To translocate on solid surfaces many bacteria use dynamic cell surface structures called type IVa pili (T4aP). T4aP undergo cycles of extension, adhesion to a surface, and retraction that generate a force sufficient to pull a cell forward. The T4aP filament is composed of thousands of copies of the major pilin. Here, using cryo-EM, we solve the structure of the T4aP of Myxococcus xanthus (T4aPMx), which has an unusual large major pilin called PilA.

For structure determination of T4aPMx, we purified T4aP from the hyperpiliated ΔpilT strain, in which T4aP are extended but not retracted, thereby allowing the purification of T4aP of sufficient purity and quantity for structural analyses. We used cryo-EM to determine the structure of the T4aPMx and obtained the structure at 3.0 Å resolution, the highest resolution so far reported for a T4aP structure. The subunits in the filament are related to each other by an azimuthal rotation of 100.7° and an axial rise per subunit of 10.0 Å, generating a right-handed 1-start helix with a pitch of ~36 Å and 3.6 subunits per turn, as determined from the power spectrum of the filaments. The filaments are ~7 nm in diameter and, in contrast to all previous T4aP structures, resemble a rather solid cylinder without the corrugation of the surface observed in other T4aP structures. The N-terminal α1-helix of PilAMx extends from residues 3 to 54 and contains the hydrophobic α1-N (aa 3 to 18) and the amphipathic α1-C (aa 24 to 54) separated by an unfolded stretch of five residues around the conserved Pro22. The large globular domain (aa 55 to 208) contains two antiparallel β-sheets, one four-stranded sheet composed of β1-4 and one three-stranded sheet composed of β1′-3′, as well as three α-helices (α2-4). Two disulfide bridges are present in the large globular domain. C95/C102 connects and likely stabilizes the region between β1 and α3. C183/C203 connects the β’-sheet to the C-terminal part of the globular domain, somewhat similar to the C-terminal D-region known from other major T4a pilins that attaches the β-sheet to the C-terminal portion of the globular domain. Within the T4aPMx the globular domain of an individual PilA monomer extensively interacts with neighboring subunits, including six different subunit–subunit interfaces, three large (N:N-3, N:N-4, N:N-1) and three small (N:N-7, N:N-2, N:N-6).

>[18x]FTLIELMIVVAIIGILAAIAIPNFIKFQARSKQSEAKTNLKALYTAQKSFFSEKDRYSDFANEIGFAPERGNRYGYRVSAAAGDCEVRNAADLPVPAAGVPCISNDSFRFGANSAIDDPTPVVARFVPQGAAGWNTTLGVQPTIADCPNCNFFAGARGNADNEATFDDWVIAGFEGSGQVGPCSEAGNVASGTPYNTRNDVACDGAAQ>[4x]MKKPNGTNGASSSLEPPPSTFQPLCHPLVEEVSKEVDGYFLQHWNFPNEKARKKFVAAGFSRVTCLYFPKALDDRIHFACR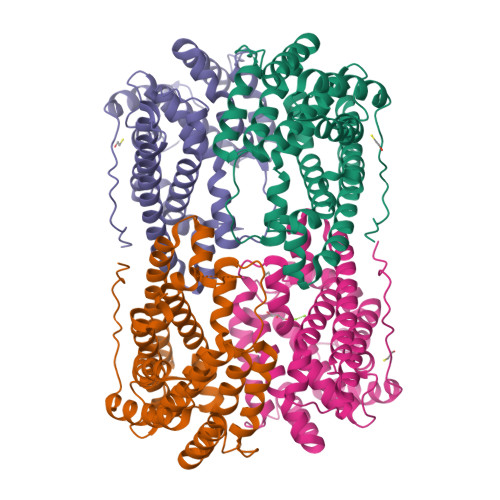LLTVLFLIDDLLEYMSFEEGSAYNEKLIPISRGDVLPDRSIPVEYIIYDLWESMRAHDREMADEILEPVFLFMRAQTDRTRARPMGLGGYLEYRERDVGKELLAALMRFSMGLKLSPSELQRVREIDANCSKHLSVVNDIYSYEKELYTSKTAHSEGGILCTSVQILAQEADVTAEAAKRVLFVMCREWELRHQLLVARLSAEGLETPGLAAYVEGLEYQMSGNELWSQTTLRYSVVVD> GDSLSIHQLAAQGELDQLKEHLRKGDNLVNKPDERGFTPLIWA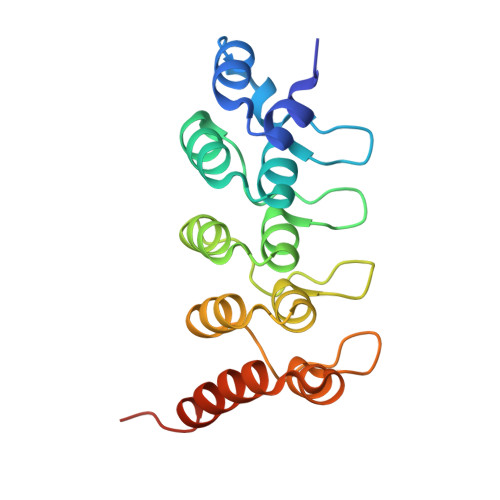SAFGEIETVRFLLEWGADPHILAKERESALSLASTGGYTDIVGLLLERDVDINIYDWNGGTPLLYAVHGNHVKCVEALLARGADLTTEADSGYTPMDLAVALGYRKVQQVIENHILKLFQSNLVPADPE>MAKKTSSKGKLPPVVSSLIPFVGSGLSFAGGPLQYTTDAYKKYGDIFTMKVFGQRLTFLVGPDAHVPFFSQGDAELSQDEPYQFSVPIFGPNVVYGADLAHRNQQLKFIAASLSTKALQSYVPLIVKEAEDFFAKWDKSGTVDIRDALAELIILTASRCLMGKEIRENLFTEVAKLYQTLDEGLLPISVFFPYLPIPAHKRRDEARLAMVRMFKKIIDERRANPEVKHNDCLQVFMDARYRGEEQALNDEEITGLMIALLFAGQHTSSVTGSWTGLLLFEANNKKKFLPGVLEEQEEIRKEFGDELTMEALNKMDKLHRCVKEALRMYPPLLFVMRKVIKPFSYKDYYVPEGDTVFVSPALSMRVEEVFPNADQYNPERFVEEDKQAQKYRFVGFGAGRHGCMGENFAYLQIKTIWSVLLRNFDIELVGELPKPDYTAMVVGPAHPCLLR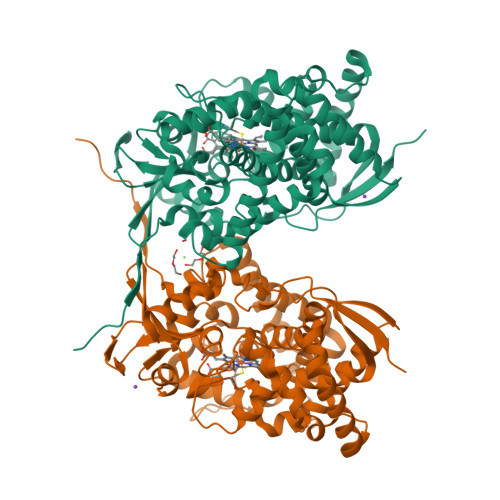YTRKHHHHHH[2x]(3M)-5-cyclobutyl-3-(1-methyl-1H-imidazol-2-yl)-1,2,4-oxadiazole 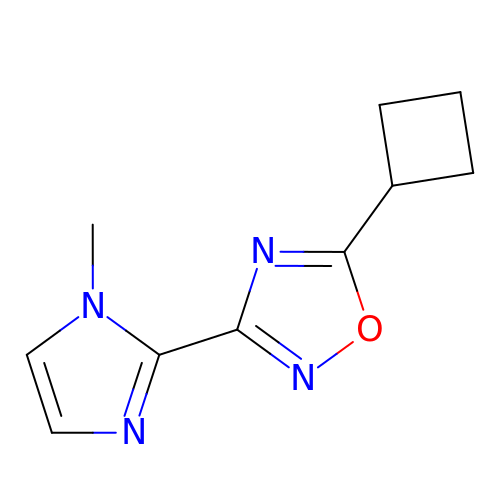| C10 H12 N4 O | OPUWQKONOBGDBJ-UHFFFAOYSA-N1-methyl-5-phenyl-1H-pyrazole-4-carboxylic acid | 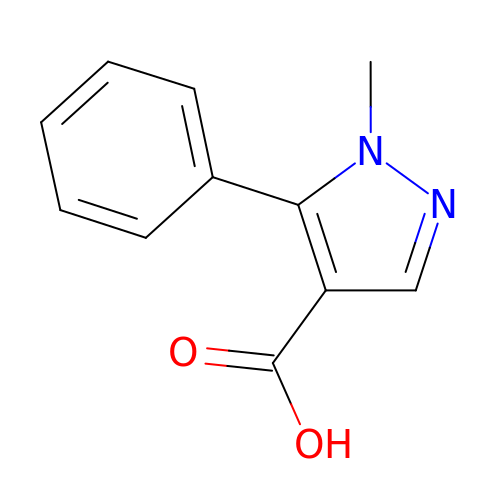C11 H10 N2 O2 | MXGOKNNGBUOAGF-UHFFFAOYSA-N GtfC-type 4,6-α-glucanotransferase (α-GT) enzymes from Glycoside Hydrolase Family 70 (GH70) are of interest for the modification of starch into low-glycemic index food ingredients. Compared to the related GH70 GtfB-type α-GTs, found exclusively in lactic acid bacteria (LAB), GtfCs occur in non-LAB, share low sequence identity, lack circular permutation of the catalytic domain, and feature a single-segment auxiliary domain IV and auxiliary C-terminal domains. The first half-reaction is α-1,4 specific cleavage of the substrate and results in a covalent enzyme-glycosyl intermediate, which is transferred with α-1,6 specificity to an acceptor substrate in the second half-reaction, leading to isomalto-/maltooligosaccharide (IMMO/IMMP) products containing α-1,6 linked units at the non-reducing end. With a limited hydrolytic activity, GbGtfC releases mainly maltose instead of glucose from amylose V or maltoheptaose substrate, synthesizing a main product containing alternating α-1,4/α-1,6 linkages instead of consecutive α-1,6 linkages.

We determined the crystal structure of GbGtfC-ΔC at a resolution of 2.25 Å from crystals containing one protomer in the asymmetric unit consisting of residues V26-K735. The crystal structure comprises domains A, B, C, and IV and is the first one representing a non-permuted GH70 enzyme. The catalytic domain A (residues 26–144 and 387–630) contains the (β/α)8 barrel also found in other GH70 enzymes, but, like in GH13 α-amylases, it starts with strand β1 and is interrupted after helix α3 by a long insertion, forming domain B, as well as the auxiliary domain IV, which is absent in GH13 enzymes. Domain B (residues 145–222 and 333–386) has the central twisted five-stranded antiparallel β-sheet also observed in other GH70 structures but is more compact, mainly due to shorter connections between the β-strands. Domain IV comprises 110 residues (223–332) and is much smaller than the corresponding domains in GtfB-type enzymes (usually about 170–180 residues); it connects to domain B via two loops that lie adjacent to each other. The crystallographic B-factors for domain IV are on average higher than for other domains, indicating that this domain may be flexible due to a hinged connection with domain B. Some of its residues hardly showed electron density, but since domain IV superimposed almost perfectly with that of the AlphaFold model, we confidently decided to include all residues of this domain in the crystal structure. Overall, the architecture of its binding groove closely resembles that of the 4,6-α-GT Lr121 GtfB, more than that of α-amylases: while the latter features a fully open binding groove, in GbGtfC, the presence of the two long loops A1 (residues 532–552) and B (residues 338–352) near the binding groove results in a tunnel-like architecture that encompasses donor subsites −2 and −3, similar to the situation in Lr121 GtfB.

> MAHHHHHHSAALEVLFQGPGYSSGPELDNRVIFQSFSLYQPYESNMYKILATKGDLLKEWGITDVWLPPAYRSFNMARYMEGYAIADRYDLGEFNQGPNNERATKYGTSDELKDMIDKLHAAGLKVQLDLVPNQLLGLNGREAVYVTRVDNNGDLFKNPYTTGLTTRIRADLYLAYTKGGGQGQAKYGYIKEWNKNYFNGTSLQGQGMGRVMTDDNGKPYRFFGPNDPRNYLPSWLEEAAAANKINTVDTYLPVDGWYAAKDAATSDQYWKPMLIHYAKDKGYLSFMSQHGFATVDDIINGDNAEIAKWTNAYIQSRPEYGFGSEERSYKNDNTGVDDQDQFLFVEENGSTKHNIHNTIHGNYEFLVGLDIDNSNPTVRKEQIHWMNWLLDTYKFDGFRIDAATHFDKQVLLDEADVRKAHFGNDLNNHLSYIESYTSKAEKFENENGNPHLTMDWALYYTLQDTLGKGTPSQKLSTIATNSVVNRSGSGSAHAIPNWSFVNNHDQEKNRVNTIMLDLYGIKTGEKYTTTPPKSFADLYDKETEKKALAIYKDDMKRVDKKYAPNNVVSQYAFLLTNKDTVPTIYYGDLYQTDASYMSKPTLYYEPITKLLKMRKAYAYGGQKITGYTSNTSPETAGQDLIASVRYGKDRYTGVAVVIGTNPKTDTTIKVDMGTKHANQVFKDATGFHSEKLVADNKGVLTIRVKGTANALVKGYLGVWVPTKDKA> MTSLEKARELLRE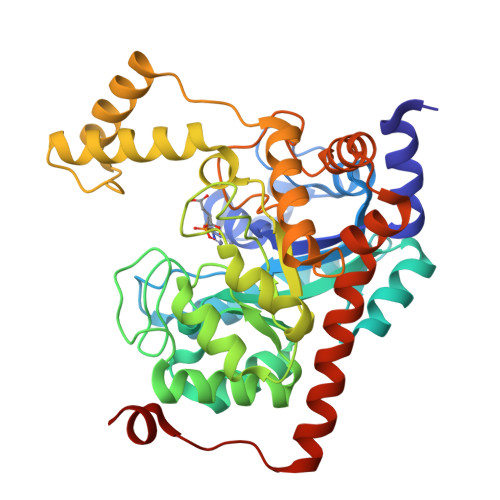FPVVDGHNDLPWALREQVRYDLDARDIAADQSAHLHTDLARLRSGGVGAQYWSVYVRSDLPGAVTATLEQIDCVRRLIDRHPGELRAALTAADMEAARAEGRIASLMGAEGGHSIDNSLATLRALYALGVRYMTLTHNDNNAWADSATDEPGVGGLSAFGREVVREMNREGMLVDLSHVAATTMRDALDTSTAPVIFSHSSSRAVCDHPRNIPDDVLERLSANGGMAMVTFVPKFVLQAAVDWTAEADDNMRAHGFHHLDSSPEAMKVHAAFEERVPRPVATVSTVADHLDHMREVAGVDHLGIGGDYDGTPFTPDGLGDVSGYPNLIAELLDRGWSQSDLAKLTWKNAVRVLDAAEDVSRGLRAARGPSNATIEQLDGTAAEQPEG>[2x]MPLPDFHVSEPFTLGIELEMQVV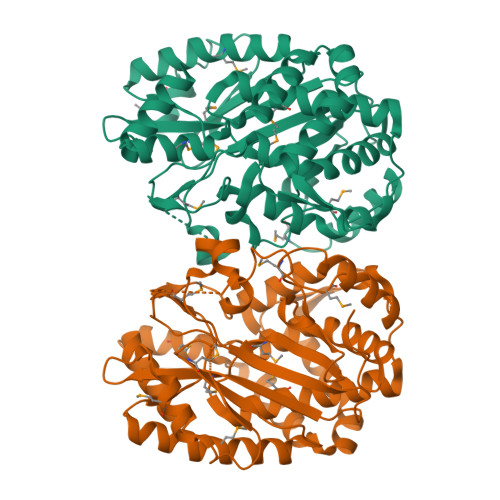NPPGYDLSQDSSMLIDAVKNKITAGEVKHDITESMLELATDVCRDINQAAGQFSAMQKVVLQAATDHHLEICGGGTHPFQKWQRQEVCDNERYQRTLENFGYLIQQATVFGQHVHVGCASGDDAIYLLHGLSRFVPHFIALSAASPYMQGTDTRFASSRPNIFSAFPDNGPMPWVSNWQQFEALFRCLSYTTMIDSIKDLHWDIRPSPHFGTVEVRVMDTPLTLSHAVNMAGLIQATAHWLLTERPFKHQEKDYLLYKFNRFQACRYGLEGVITDPHTGDRRPLTEDTLRLLEKIAPSAHKIGASSAIEALHRQVVSGLNEAQLMRDFVADGGSLIGLVKKHCEIWAGD> MMVFQSFILGNLVSLCMKIINSVVVVGLYYGFLTTFSIGPSYLFLLRARVMDEGEEGTEKKVSATTGFIAGQLMMFISIYYAPLHLALGRPHTITVLALPYLLFHFFWNNHKHFFDYGSTTRNEMRNLRIQCVFLNNLIFQLFNHFILPSSMLARLVNIYMFRCNNKMLFVTSSFVGWLIGHILFMKWVGLVLVWIQQNNSIRSNVVIRSNKYKFLVSELRNS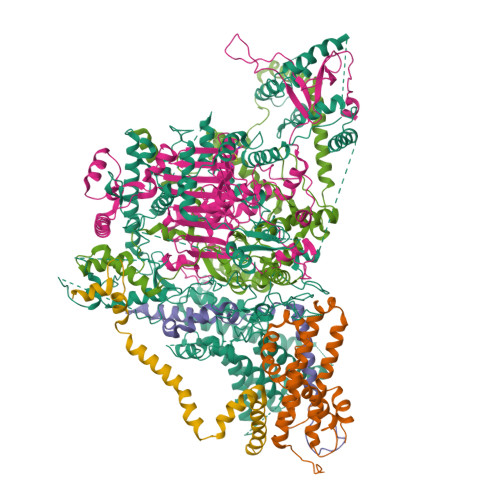MARIFSILLFITCVYYLGRIPSPIFTKKLKGTSETGGTKQDQEVSTEEAPFPSLFSEEGEDLDKIDEMEEIRVNGKDKINKDDEFHVRTYYNYKTVSENLYGNKENSNLEFFKIKKKEDHFLWFEKPFVTLVFDYKRWNRPNRYIKNDKIENIVRNEMSQYFFYTCQSDGKERISFTYPPNLSTFFEMIQKRIPSFTKEKKTFDQVSTYWSLIHEEKRENLKKEFLNRIEALDKEWSVENILEKTTRFCYNEAKKEYLPKIYDPFLHGISRGRIKKLPPFQIITETYRKNNLGGSWINKIHGLLLKINYKKFEQTIEKFNRKSLSIEKKLSFFSEPQQEEKINSEEEIKTFKFLFDIVRTDSNDQTLIKNFMDFPEINKKVPRWSYKLISELEELEGENEENVPMEPGIRSRKAKRVVVFTDKEPHGEIYTNLKDNQNSDQNDEMALIRYSQQSDFRREIIKGSMRSQRRKTVIWEFFQAKVHSPLFFDRIDKLFFFSFDIWGLKKKIIKNFIWKKKIDKKEEEQSKREETRRIEIAETWDSFLFAQIIRGSLLVTQSILRKYIILPLLIIIKNSVRMLLFQFPEWSQDLKDWKREMHVKCTYNGVQLSETEFPRNWLTDGIQIKILFPFYLKPWHKSKFQASQKARLKKTKDKGEKNDFCFLTVWGMETELPFGSAQRKPSFFEPISKELKKRIKKLKKKSFVVLKIFKERAPIFLKVAKETKNWILKNFIFIKGISKRNLIPLFGPREIYELNEPKKDSIISNQMIHELSVQNKSLEWTNSSLSEKKIKNLIDRKKTIRNQIEEISKEKQNLTNSCTKLRYDSKIIESSKKIWQTFKRKNTRLIRKSIFFFKFCIEQMSIAIFLGIINIPRITTQLFFESTKKILDKYIYKNEENGEKKKNTLYFISTIKNLISNKKKMSYDLCSLSQAYVFYKLSQIKVSNFCKLKAVLEYNICITSFFVKNKIKVFFQEHGIFHYELKNKTFLNSEVNQWKNWLRSQYQYNLPQISWARLVTQNWKNKINKDSLVLNPSLTKEDSYEKKKFDNYKKQKFFEADSLLNPKHNVKKDSIYNLFCYKSIHSTEKNFDMSIGIALDNCLVSSFLEKYNIRGMGEIRHRKYLDWRILNFWFTKKVTIEPWVDTKSKKKYINTKVQNYQKIDKITQTDLANKKRNFFDWMGMNEEILNQRITNFEFFFFPEFFLFSSTYKMKPWVIPIKLLLLNFNENINVNKKIIRKKKGFIPSNEKESLRFYNLNKEEKESAGQVELESDKETKRNPEAARLNQEKNIEENFAESTIKKRKNKKQYKSNTEAELDLFLTRYSRFQLRWNCFFNQKILNNVKVYCLLVRLNNPNEIAVSSIERGEMSLDILMIEKNFTFAKLMKKGILIIEPVRLSVQNDGQLIIYRTIGISLVHKNKHKISKRYKKKSYINKKFFEKSITKYQNKTVNKKKNNYDFFVPEKILSPKRRREFRILICFNLKKKNARDTNSRFDKNIQNLTTVLHKKKDLDLDKDKNNLINLKSFLWPNFKLEDLACMNRYWFNTTNGNHFSMIRIRMYTRFPIP;> MITGYSTPSAHVLMSSRAFKSSSYRAAAGQTQHYLARSSLPVVKNSWGSPPSPFNELPRVSRGVPLSYLSASSSLLLNGEQGSLSGTLPVLPVRRKTLLTPRASKDVPSSFRFPPMTKKPQWWWRTLACLPYLMPLHETWMYAETAYHLHPFLEDFEFLTYPFLGAIGRLPSWFLMAYFFVAYLGIVRRKEWPHFFRFHVVMGMLLEIALQVIGTVSKWMPLGVYWGKFGMHFWTAVAFAYLFTVLESIRCALAGMYADIPFVCDAAYIQIPYD;> MEKYFGNAYRGDPGVPHADADRFVNIWIGSAAFSVLTWVNPYMWQLSNQFNYHDKWMLFEQYHWKKARAKKQPYEFKWNKIPKEVRDSYYYNWPVYFP;> MANEELTESQQQEDPSQQLPNADEEKGSDSDSNSDSDASSQSSGDDFYISESENEAEGDNTIFNYVRPSDIPPDPNANPETNIRRFNRVLDGKRVKRMQEEEEDKYTFYEDLFDFPRDPERWKEQDLREIWADGPLEMTKPGWDPAWADEDDWDVVNDEIQEGRDPGIQPFYVPYRKPYPAIPDNHYDIENAKGVVEELDRIEEFLQWVSYIFPDGSSYEGTVWDDLAQGKGVYIAENGLVRYEGEWLQNDMEGHGVIDVDIPDIEPIPGSKLEAKMRAEGRIIKRDYMTPEDRKWLEMDVEDSVALTDGNFQVPFYENEEWVTQFGEKPEKGRYRYAGQWKHSRMHGCGVYEVNERILYGRFYFGELLEEEHGCTVDICALHSGLAEVAAAKARMFVNKPDGMIREERGPYGDPQHPYFYEEDDVWMAPGFINQFYEVPEYWETYVGEVDQEREMWLNSFYKAPLRLPMPAELEHWWENVEVTPEFVLLNKEPEPDPNDPSKLVQKEDPVILHTPTGRIINYVEDEKHGIRLFWQPPLEEGEEVDPSKVEFLPLGFDEFYGKEVVVKKEHPIKSFVLGIEKSVKPMLDGLEKWTEEKKKAYEERKEMIQQELELVEAEICLEEAIEDMDEELKKKEQEEEKKTEMGLTEEDEDVLVPVYKEEKVVTAKEKIQENKQEEKYKDDDDEDDDDGDDDDDDDDDDDLGPSSFGSADKGRRNSPFSSSSLSFASCTLFPAVQSRLESSFLAWKQHRAEPSKVNTGIIKGADTASASIHFPPLSSNNARLKMGKVANRGCVQRSYGSSRSQSQLMSLSRLLSCNASSSSSPPDSSSSEYLKDSGLWETPVGDMSVVLSLQIQTKCSDLFAETPAVS;> MSSMNFNPFQNWFEKPPNPVPSINFVSLADSFFPKSQSPNFASIGLPKFSKKSPKPETAGTDEPGPYKQIAEQFLWECENIPDYRHTPEVDKLLNEDPVFEKKENPSTEEIEAEQKWWESFRASPVVQFMTRAEEIADDMNKMELEDNDTPYRKEDKDYWRAIPHVPGFDGRPMPRKAIKSKEESDDKFWDFMKQFLFGLWGFRQRPYPPGRPIDVAQAIGYKRLEKRYYDFIMKTGGWWYKDRLGRSRGPCEIITLKTAYGAGIIDRDTFIWGEDMDEWAPIHMVYGLEPAIATWEVRLGAAATAFLHKLQKGIPPWVPLKGREPKTYKQLQKEAIESKKRDMAVLEANGGVWPGVRTPSHALFLWASGSELTTVLESDHMPNKFIPKQLRLELAKVIPGLRPWEVISIEQAMDQISYGGEWYREPLGTYTTGPPYIREWNRSVMRLFRIFYNLSVRVGQKLERTVPGFDTIMDKVQKDYDKRIARRMKRREEELREEDLKHYSGRTDEDEEEEEEEDDDSNSKKD;> MSFTQANCFRPSYYPARITRPNCISSVPIRSSVRFDHFPRTSFTLRATAAVSTQFSPLLDHRRRLPTGKSKQSSAVCLFGGKDKPDGSDEISPWKAIEKAMGKKSVEDMLREQIQKKDFYDTDSGGNMPPRGGGSGGGGGNGEERPEGSGGEDGGLAGIADETLQVVLATLGFIFLYTYIITGEELVKLARDYIRFLMGRPKTVRLTRAMDSWNGFLEKMSRQRVYDEYWLEKAIINTPTWYDSPEKYRRVIKAYVDSNSDEAYVESNSDEVSY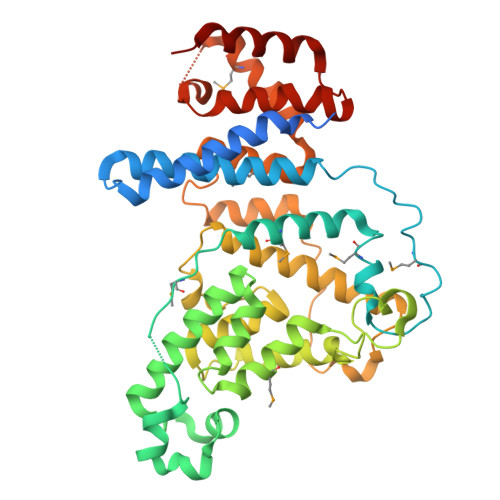> GSMELSPTYQTERFTKFSDTLKEFKIEQNNEQNPIDPFNIIREFRSAAGQLALDLANSGDESNVISSKDWELEARFWHLVELLLVFRNADLDLDEMELHPYNSRGLFEKKLMQDNKQLYQIWIVMVWLKENTYVMERPKNVPTSKWLNSITSGGLKSCDLDFPLRENTNVLDVKDKEEDHIFFKYIYELILAGAIDEALEEAKLSDNISICMILCGIQEYLNPVIDTQIANEFNTQQGIKKHSLWRRTVYSLSQQAGLDPYERAIYSYLSGAIPNQEVLQYSDWESDLHIHLNQILQTEIENYLLENNQVGTDELILPLPSHALTVQEVLNRVASRHPSESEHPIRVLMASVILDSLPSVIHSSVEMLLDVVKGTEASNDIIDKPYLLRIVTHLAICLDIINPGSVEEVDKSKLITTYISLLKLQG>[2x]SQKVEKTVIKNETGTISIS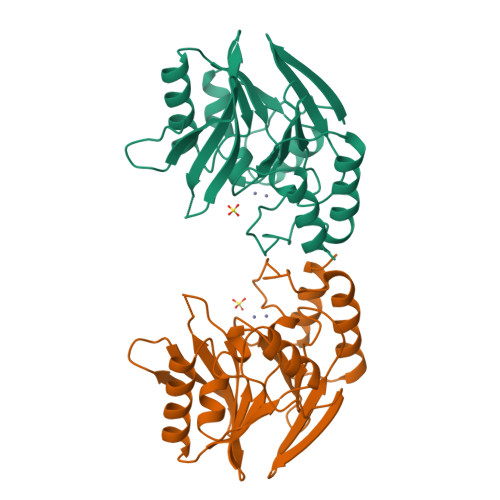QLNKNVWVHTELGSFNGEAVPSNGLVLNTSKGLVLVDSSWDDKLTKELIEMVEKKFQKRVTDVIITHAHADRIGGIKTLKERGIKAHSTALTAELAKKNGYEEPLGDLQTVTNLKFGNMKVETFYPGKGHTEDNIVVWLPQYNILVGGCLVKSTSAKDLGNVADAYVNEWSTSIENVLKRYRNINAVVPGHGEVGDKGLLLHTLDLLK> GP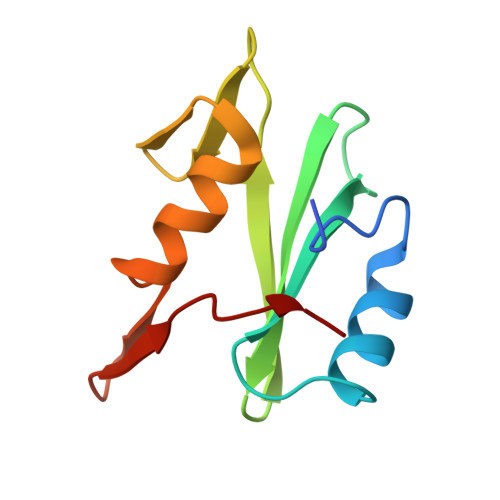LGSEWYYGNVTRHQAECALNERGVEGDFLIRDSESSPSDFSVSLKASGKNKHFKVQLVDNVYCIGQRRFHTMDELVEHYKKAPIFTSEHGEKLYLVRALQ> KDDMKAAEQYQGAASAVDPAHVVRTNGAPDMSESEFNEAKQIYFQRCAGCHGVLRKGATGKPLTPDITQQRGQQYLEALITYGTPLGMPNWGSSGELSKEQITLMAKYIQHTPPQPPEWGMPEMRESWKVLVKPEDRPKKQLNDLDLPNLFSVTLRDAGQIALVDGDSKKIVKVIDTGYAVHISRMSASGRYLLVIGRDARIDMIDLWAKEPTKVAEIKIGIEARSVESSKFKGYEDRYTIAGAYWPPQFAIMDGETLEPKQIVSTRGMTVDTQTYHPEPRVAAIIASHEHPEFIVNVKETGKVLLVNYKDIDNLTVTSIGAAPFLHDGGWDSSHRYFMTAANNSNKVAVIDSKDRRLSALVDVGKTPHPGRGANFVHPKY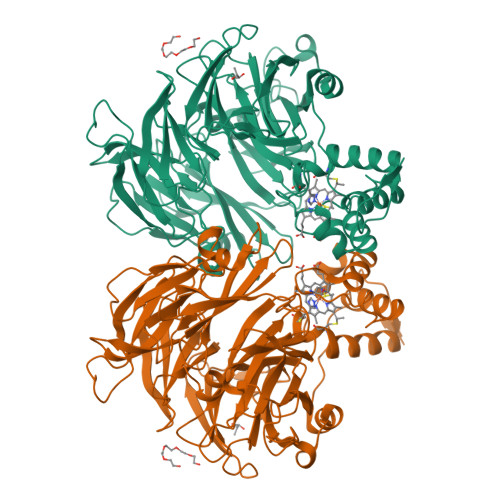GPVWSTSHLGDGSISLIGTDPKNHPQYAWKKVAELQGQGGGSLFIKTHPKSSHLYVDTTFNPDARISQSVAVFDLKNLDAKYQVLPIAEWADLGEGAKRVVQPEYNKRGDEVWFSVWNGKNDSSALVVVDDKTLKLKAVVKDPRLITPTGKFNVYNTQHDVY> MKRIPRKTKGKSSGKGNDSTERSDDGSSQLRDKQNNKAGPATTEPGTSNREQYRARPGIASVQRATESAELPMKNNDEGTPDKKGNTRGDLVNEHSEAKDEADEATQKQAKDTDKSKAQVTYSDTGINNANELSRSGNVDNEGGSNQKPMSTRIAEATSAIVSKHPARVGLPPTASSGHGYQCHVCSAVLFSPLDLDAHVASHGLHGNMTLTSSEIQRHITEFISSWQNHPIVQVSADVENKKTAQLLHADTPRLVTWDAGLCTSFKIVPIVPAQVPQDVLAYTFFTSSYAIQSPFPEAAVSRIVVHTRWASNVDFDRDSSVIMAPPTENNIHLFKQLLNTETLSVRGANPLMFRANVLHMLLEFVLDNLYLNRHTGFSQDHTPFTEGANLRSLPGPDAEKWYSIMYPTRMGTPNVSKICNFVASCVRNRVGRFDRAQMMNGAMSEWVDVFETSDALTVSIRGRWMARLARMNINPTEIEWALTECAQGYVTVTSPYAPSVNRLMPYRISNAERQISQIIRIMNIGNNATVIQPVLQDISVLLQRISPLQIDPTIISNTMSTVSESTTQTLSPASSILGKLRPSNSDFSSFRVALAGWLYNGVVTTVIDDSSYPKDGGSVTSLENLWDFFILALALPLTTDPCAPVKAFMTLANMMVGFETIPMDNQIYTQSRRASAFSTPHTWPRCFMNIQLISPIDAPILRQWAEIIHRYWPNPSQIRYGAPNVFGSANLFTPPEVLLLPIDHQPANVTTPTLDFTNELTNWRARVCELMKNLVDNQRYQPGWTQSLVSSMRGTLDKLKLIKSMTPMYLQQLAPVELAVIAPMLPFPPFQVPYVRLDRDRVPTMVGVTRQSRDTITQPALSLSTTNTTVGVPLALDARAITVALLSGKYPPDLVTNVWYADAIYPMYADTEVFSNLQRDMITCEAVQTLVTLVAQISETQYPVDRYLDWIPSLRASAATAATFAEWVNTSMKTAFDLSDMLLEPLLSGDPRMTQLAIQYQQYNGRTFNVIPEMPGSVIADCVQLTAEVFNHEYNLFGIARGDIIIGRVQSTHLWSPLAPPPDLVFDRDTPGVHIFGRDCRISFGMNGAAPMIRDETGMMVPFEGNWIFPLALWQMNTRYFNQQFDAWIKTGELRIRIEMGAYPYMLHYYDPRQYANAWNLTSAWLEEITPTSIPSVPFMVPISSDHDISSA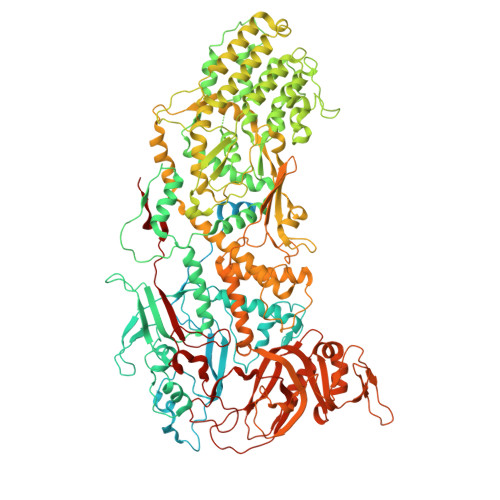PAVQYIISTEYNDRSLFCTNSSSPQTIAGPDKHIPVERYNILTNPDAPPTQIQLPEVVDLYNVVTRYAYETPPITAVVMGVP>GESELSSNPAASAGASLEPPAAPAPGEDNPAGAGGAAVAGAAGGARRFLCGVVEGFYGRPWVMEQRKELFRRLQKWELNTYLYAPKDDYKHRMFWREMYSVEEAEQLMTLISAAREYEIEFIYAISPGLDITFSNPKEVSTLKRKLDQVSQFGCRSFALLFDDIDHNMCAADKEVFSSFAHAQVSITNEIYQYLGEPETFLFCPTEYCGTFCYPNVSQSPYLRTVGEKLLPGIEVLWTGPKVVSKEIPVESIEEVSKIIKRAPVIWDNIHANDYDQKRLFLGPYKGRSTELIPRLKGVLTNPNCEFEANYVA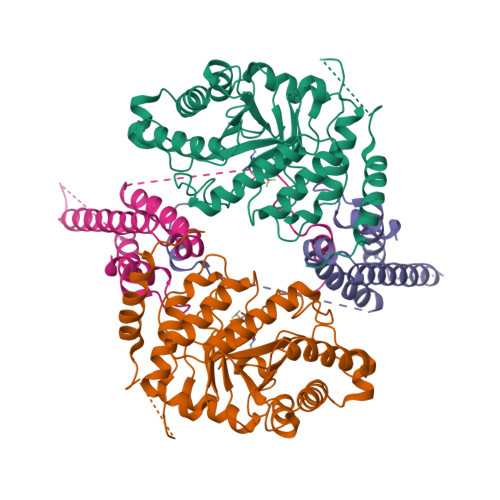IHTLATWYKSNMNGVRKDVVMTDSEDSTVSIQIKLENEGSDEDIETDVLYSPQMALKLALTEWLQEFGVPHQYSSR[4x];>[4x]MTLEDLQLLADLFYLPYEHGPKGAQMLREFQWLRANSSVVSVNCKGKDSEKIEEWRSRAAKFEEMCGLVMGMFTRLSNCANRTILYDMYSYVWDIKSIMSMVKSFVQWLGCRSHSSAQFLIGDQEPWAFRGGLAGEFQRLLPIDGANDLFFQPHHHHHHHH>[4x]SVAEINAQYYQQESAKLRQQIISIQNSNRQ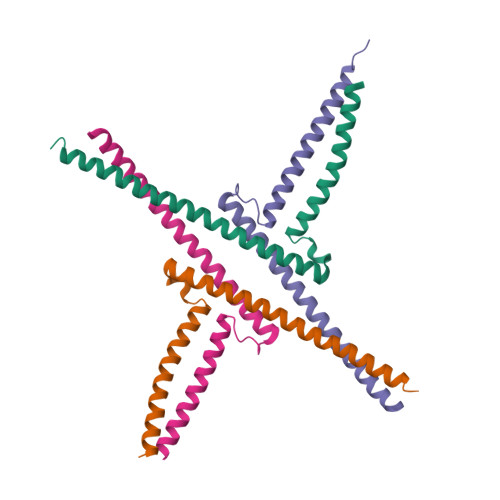LMGETIGSMSPKELRNLEGRLERSITRIRSKKNELLFSEIDYMQKREVDLHNDNQILRAKIAENRN;>PNVPSREALAVELSSQQEYLKLKERYDALQRTQRNLLGEDLGPLSTKELESLERQLDSSLKQIRALRTQFMLDQLNDLQSKERMLTETNKTLRLRLAD[4x]> GTVPPFIQPFEFPRFSIGQRVFIPCVVVSGDLPITITWQKDGRPIPGSLGVTIDNIDFTSSLRISNLSLMHNGNYTCIARNEAAAVEHQSQLIVRVPPKFVVQPRDQDGIYGKAVILNCSAEGYPVPTIVWKFSKGAGVPQFQPIALNGRIQVLSNGSLLIKHVVEEDSGYYLCKVSNDVGADVSKSMYLTVKIPAMITSYPNTTLATQGQKKEMSCTAHGEKPIIVRWEKEDRIINPEMARYLVSTKEVGEEVISTLQILPTVREDSGFFSCHAINSYGEDRGIIQLTVQEELENLYFQGSHHHHHH

Here, we present the use of the GlycoDelete (GD) HEK cell line for protein crystallization, which produces homogeneous mature-like trisaccharide glycan stubs. The GD cell line is derived from the HEK293S MGAT1−/− cell line and has been transformed with Golgi-resident EndoT (an endo-β-N-acetyl­glucosaminidase similar to EndoH). This enzyme processes the Man5GlcNAc2 glycans, allowing the NG to be further processed by native Golgi-resident enzymes to generate mature-like glycans consisting of one GlcNac (which can be fucosylated), one galactose (Gal) and one sialic acid (Neu5Ac). The glycan stubs do not need further enzymatic processing, and we show that for heavily glycosylated fragments of human colony-stimulating factor 1 receptor (CSF-1R), murine IL-12B and human Down syndrome cell-adhesion molecule (DSCAM) the NG modifications facilitate the production of diffraction-quality crystals.

Down syndrome cell-adhesion molecule (DSCAM) is a cell-surface glycoprotein with an extensive ectodomain consisting of ten immunoglobulin domains and six fibronectin domains. To further characterize the portion of the ectodomain of human DSCAM that interacts with netrin, we produced a truncated fragment consisting of immunoglobulin domains Ig7, Ig8 and Ig9. Wild-type-derived rod-shaped crystals were obtained of significant size and good morphology, but X-ray diffraction screening on the microfocus beamline P14 only resulted in diffraction patterns to ∼8 Å resolution. GD-derived crystals from the initial condition diffracted to 2.5 Å resolution and further optimization of the conditions resulted in a complete data set from a single crystal at 1.85 Å resolution. The crystal structure of human DSCAMIg7–Ig9 contains one molecule in the asymmetric unit. The fragment corresponds to three immunoglobulin (Ig)-type C2 domains, each consisting of two layers of antiparallel β-sheets held together by a conserved disulfide bond. Clear electron density for the glycan chains was observed in all three Ig domains at residues Asn666, Asn710, Asn748 and Asn795. The predicted glycan at Asn658 was not observed in the electron density. An analysis of the buried surface areas of all of the contacts occurring in the crystal lattice reveals that the most extensive protein interface is formed between Ig7 and a symmetry-related Ig7 domain (830 Å2). When this protein interface is compared with the Ig7–Ig7 interface observed in available Drosophila DSCAM crystal structures, it is remarkably similar. We conclude therefore that the rigidity of the glycan stub substantially contributes to crystal formation, but without disrupting the biologically relevant dimerization of the receptor fragment.> SFVDHPPDWLEEVGEGLREFLGLEAGPPKPKPNQQHQDQARGLVLPGYNYLGPGNGLDRGEPVNRADEVAREHDISYNEQLEAGDNPYLKYNHADAEFQEKLADDTSFGGNLGKAVFQAKKRVLEPFGLVEEGAKTAPTGKRIDDHFPKRKKARTEEDSKPSTSSDAEAGPSGSQQLQIPAQPASSLGADTMSAGGGGPLGDNNQGADGVGNASGDWHCDSTWMGDRVVTKSTRTWVLPSYNNHQYREIKSGSVDGSNANAYFGYSTPWGYFDFNRFHSHWSPRDWQRLINNYWGFRPRSLRVKIFNIQVKEVTVQDSTTTIANNLTSTVQVFTDDDYQLPYVVGNGTEGCLPAFPPQVFTLPQYGYATLNRDNTENPTERSSFFCLEYFPSKMLRTGNNFEFTYNFEEVPFHSSFAPSQNLFKLANPLVDQYLYRFVSTNNTGGVQFNKNLAGRYANTYKNWFPGPMGRTQGWNLGSGVNRASVSAFATTNRMELEGASYQVPPQPNGMTNNLQGSNTYALENTMIFNSQPANPGTTATYLEGNMLITSESETQPVNRVAYNVGGQMATNNQSSTTAPATGTYNLQEIVPGSVWMERDVYLQGPIWAKIPETGAHFHPSPAMGGFGLKHPPPMMLIKNTPVPGNITSFSDVPVSSFITQYSTGQVTVEMEWELKKENSKRWNPEIQYTNNYNDPQFVDFAPDSTGEYRTTRPIGTRYLTRPL;> MASHHHHHHVSAGESVQITLPKNEVQLNAYVLQEPPKGETYTYDWQLITHPRDYSGEMEGKHSQILKLSKLTPGLYEFKVIVEGQNAHGEGYVNVTVKPEPRKNRPPIAIVSPQFQEISLPTTSTVIDGSQSTDDDKIVQYHWEELKGPLREEKISEDTAILKLSKLVPGNYTFSLTVVDSDGATNSTTANLTVNKAVD

Adeno-Associated Virus (AAV) is a small (~25 nm diameter) non-enveloped single-stranded DNA virus in the Parvoviridae family (genus Dependoparvovirus). The icosahedral proteinaceous shell is composed of three capsid proteins. These proteins (named VP1, VP2 and VP3) share an open reading frame and differ only in their N-terminal residues. We use a high resolution (2.5 Å) cryo-EM structure to analyze details of the molecular interactions that are presumed to be key to efficient infection and are likely to be relevant to serotype-specific tissue tropism.

However, in the receptor bound reconstruction, a PKD domain of AAVR was bound, at its C-terminal end, on the side of each three-fold AAV5 proximal spike. The PKD N-terminal end was disordered and pointing toward the five-fold axis of symmetry. The resolution of the reconstruction is sufficient to distinguish side chains that identify the domain as PKD1. PKD1 binds to AAV5 near the 3-fold symmetry axis spike, primarily to two of the variable regions (VR) in the AAV sequence that have previously been highlighted, namely VR-VII and a segment containing VR-IX. The C–D and E–F loops in the beta sandwich that makes up PKD1 contain most of the binding interactions. The two AAVR residues, R353 and H351, are of particular importance due to their potential for polar interactions with AAV5. AAVR R353, extends from the end of PKD1 into a polar pocket between the AAV5 VR-VII and VR-IX loops. The positively charged R353 guanidinium is extended towards a negatively charged region of the viral surface near AAV5 E544. Similarly, AAVR H351 interacts with a charged region of the AAV5 surface. Instead they involve hydrophobic contacts formed by AAVR L376 and AAV5 Y542, L543 and A540.> MAVPFVEDWDLVQTLGEGAYGEVQLAVNR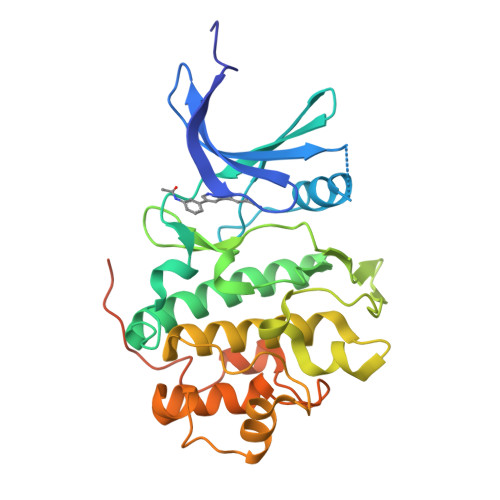VTEEAVAVKIVDMKRAVDCPENIKKEICINKMLNHENVVKFYGHRREGNIQYLFLEYCSGGELFDRIEPDIGMPEPDAQRFFHQLMAGVVYLHGIGITHRDIKPENLLLDERDNLKISDFGLATVFRYNNRERLLNKMCGTLPYVAPELLKRREFHAEPVDVWSCGIVLTAMLAGELPWDQPSDSCQEYSDWKEKKTYLNPWKKIDSAPLALLHKILVENPSARITIPDIKKDRWYNKPLKKGAKRPRVTSGGVSESPSGGHHHHHHHH>GPGSKPFSLPILTLSELTNSRFPVPIDSLFTAQNNVLQVQCQNGRCTLDGELQGTTQLLPSGICAFRGRVTAETDHRDKWHMQLQNL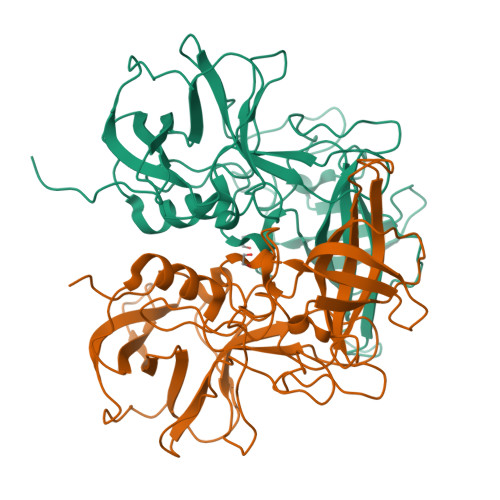NGTTYDPTDDVPAPLGTPDFKGVVFGVASQRNVGNDAPGSTRAHEAVISTYSPQFVPKLGSVNFRSNDNDFQLQPTKFTPVGINDDGDHPFRQWELPDYSGLLTLNMNLAPPVAPNFPGEQLLFFRSFVPCSGGYNQGIVDCLIPQEWIQHFYQESAPSQSDVALIRYVNPDTGRTLFEAKLHRSGYITVAHSGDYPLVVPANGYFRFDSWVNQFYSLAPM[2x]>[4x]YPPSMDWRKKGNFVSPVKNQGSCGSCWTFSTTGALESAVAIATGKMLSL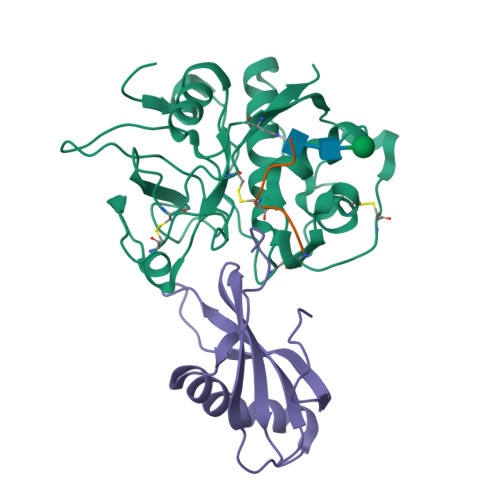AEQQLVDCAQNFNNHGCQGGLPSQAFEYIRYNKGIMGEDTYPYKGQDDHCKFQPDKAIAFVKDVANITMNDEEAMVEAVALYNPVSFAFEVTNDFLMYRKGIYSSTSCHKTPDKVNHAVLAVGYGEENGIPYWIVKNSWGPQWGMNGYFLIERGKNMCGLAACASYPIPLV;>MIPGGLSEAKPATPEIQEIVDKVKPQLEEKTNETYGKLEAVQYKTQVVAGTNYYIKVRAGDNKYMHLKVFKSLPGQNEDLVLTGYQVDKNKDDELTGF[4x];>EPQNCSAT[4x]>[4x]MRQTEDVAEVLNRCASSNWSERKEGLLG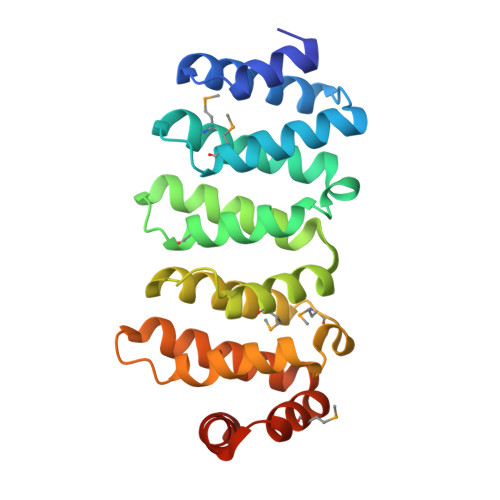LQNLLKNQRTLSRIELKRLCEIFTRMFADPHGKVFSMFLETLVDFIQVHKDDLQDWLFVLLTQLLKKMGADLLGSVQAKVQKALDITRESFPNDLQFNILMRFTVDQTQTPSLKVKVAILKYIETLAKQMDPRDFTNSSETRLAVSRVITWTTEPKSSDVRKAAQSVLISLFELNTPEFTMLLGALPKTFQDGATKLLHNHLRN> MNTEIISPHHYVYPNTTTLKNKYGIKNLNAFLEKCSHDTAKAMINLREESLPEYFDTAYLCHIHQQLFKNTFEWAGYLRHIPFTFADGTTAAMPEMKRTGWKNAFAIGDEIQEGLQRLDQTLAEKNNLQGLTREEFNSEAIELFNSLNQLHPFREGNGRTQRLFFENLAKAAGHQLNFSLITKERMMVASVAVAENGDLEPMQHLFEDISNPEKIRLLKEFMHTMKNTGRNVNDRPVMVAKEGETYTGTYRGAGLEGFALNVKGAYIIGNIDHLPPEQLKILKPGDKITFTAPKAH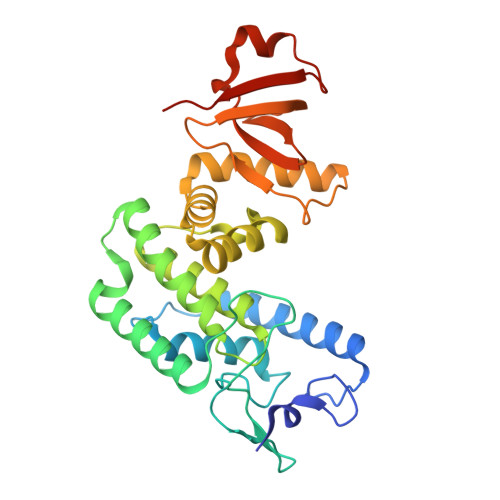HHHHH>KVELVFVPGPGIGHLSTALQIADLLLRRDHRLSVTVLSIPLPWEAKTTTQPESLFPSSTTTTTSRIRFISLPQRPLPDDAKGPFQFQAVFETQKQNVKEAVAKLSDSSILAGLVLDMFCVTMVDVAKQLGVPSYVFFTSSAGYLSFTSHLQDLSDRHGKETQQLMRSDVEIAVPGFTNPVPGKVIPGVYFNKNMAEWLHDCARRFRETNGILVNTFSELESQVMDSFSDATAASQFPAVYAVGPILSLNKNTSAASSESQSGDEILKWLDQQPPSSVVFLCFGSKGSLNPDQAREIAHALERSGHRFVWSLRQPSPKGKFEKPIEYDNIEDVLPEGFLDRTAEMGRVIGWAPQVEILGHPATGGFVSHCGWNSTLESLWYGVPIATWPMYAEQHFNAFEMGVELGLAVGISSESSIEEGVIVSAEKIEEGIRKLMGGGGGGGGGEVRKLVKAKSEESR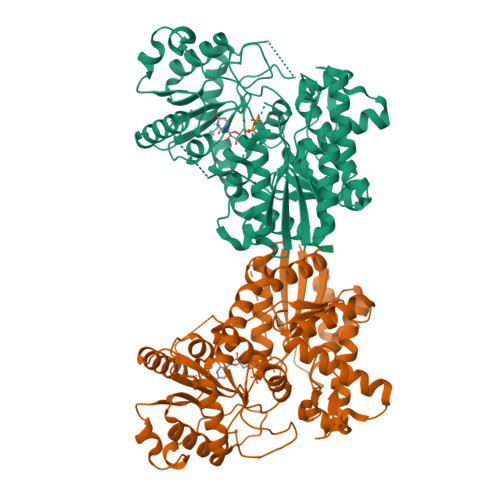KSVMEGGSSFTSLNRFIDEVMKSPF[2x]> RDLVIQNEYLRARFDPNTGLLMELENLEQNLLLPVRQAFYWYNASTGNNLSSQASGAYIFRPNQNKPLFVSHWAQTHLVKASLVQEVHQNFSAWCSQVVRLYPRQRHLELEWTVGPIPVGDGWGKEVISRFDTALATRGLFYTDSNGREILERRRNYRPTWKLNQTEPVAGNYYPVNSRIYITDGNMQLTVLTDRSQGGSSLRDGSLELMVHRRLLKDDARGVGEPLNKEGSGLWVRGRHLVLLDKKETAAARHRLQAEME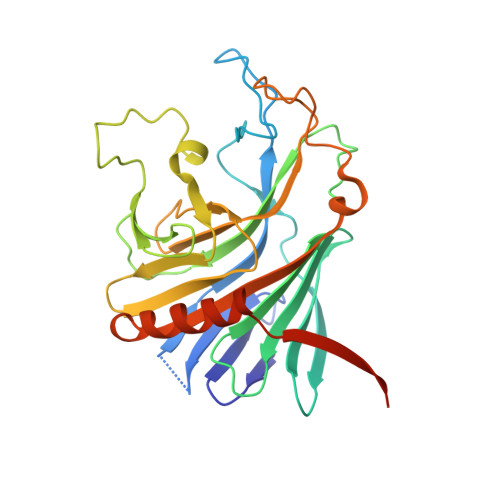VLAPQVVLAQGGGARYRLEKA Human Epidermal growth factor Receptor 4 (HER4 or ERBB4) carries out essential functions in the development and maintenance of the cardiovascular and nervous systems. HER4 activation is regulated by a diverse group of extracellular ligands including the neuregulin (NRG) family and betacellulin (BTC), which promote HER4 homodimerization or heterodimerization with other HER receptors. Important cardiovascular functions of HER4 are exerted via heterodimerization with its close homolog and orphan receptor, HER2. Here, we report cryo-EM structures of near full-length HER2/HER4 heterodimers and full-length HER4 homodimers bound to NRG1β and BTC.

We used this set of interface mutations to enrich for the fraction of functional HER2-G778D-V956R/HER4-I712Q heterodimers in large-scale purification for structural studies. Focused data processing on the ectodomains resulted in reconstructions of the NRG1β- and BTC-bound HER2/HER4 heterodimers at 3.3 Å and 4.3 Å resolution, respectively. We present here the first cryo-EM reconstructions of both the homodimer and heterodimer complexes of the HER4 receptor in its full-length form, bound to two different high-affinity HER4 cognate growth factors, NRG1β and BTC. This is also the first time that a betacellulin growth factor has been resolved bound to a HER receptor. Despite the diverse sequences of the NRG1β and BTC ligands, the larger-scale domain conformation of the HER2/HER4 heterodimers stabilized by each ligand is identical with only small differences in the ligand binding pockets. Due to the lower resolution of the HER2/HER4/BTC complex, we cannot exclude the possibility of differences in side-chain arrangements between the two structures. However, we attribute the lower resolution to variability in data collection on GO grids, rather than differences in conformational heterogeneity of HER2/HER4/BTC. HER2 and HER4 dimerization arms are resolved in both NRG1β and BTC-bound HER2/HER4 complexes. Extensive 3D variability and 3D classification analysis of the HER2/HER4/NRG1β and HER2/HER4/BTC datasets did not reveal any defined conformational heterogeneity within domains IV or dimerization arm regions. N-linked glycosylation is also resolved in the cryo-EM maps of the HER2/HER4 heterodimers (NRG1β and BTC bound), with HER4 glycosylation patterns being the same as seen in homodimers. However, in contrast to the HER4 homodimers, we do not observe continuous density connecting the two heterodimer monomers indicating that glycan-mediated interfaces seen in HER4 homodimers cannot be established in HER2/HER4 heterodimers.

> QSVCAGTENKLSSLSDLEQQYRALRKYYENCEVVMGNLEITSIEHNRDLSFLRSVREVTGYVLVALNQFRYLPLENLRIIRGTKLYEDRYALAIFLNYRKDGNFGLQELGLKNLTEILNGGVYVDQNKFLCYADTIHWQDIVRNPWPSNLTLVSTNGSSGCGRCHKSCTGRCWGPTENHCQTLTRTVCAEQCDGRCYGPYVSDCCHRECAGGCSGPKDTDCFACMNFNDSGACVTQCPQTFVYNPTTFQLEHNFNAKYTYGAFCVKKCPHNFVVDSSSCVRACPSSKMEVEENGIKMCKPCTDICPKACDGIGTGSLMSAQTVDSSNIDKFINCTKINGNLIFLVTGIHGDPYNAIEAIDPEKLNVFRTVREITGFLNIQSWPPNMTDFSVFSNLVTIGGRVLYSGLSLLILKQQGITSLQFQSLKEISAGNIYITDNSNLCYYHTINWTTLFSTINQRIVIRDNRKAENCTAEGMVCNHLCSSDGCWGPGPDQCLSCRRFSRGRICIESCNLYDGEFREFENGSICVECDPQCEKMEDGLLTCHGPGPDNCTKCSHFKDGPNCVEKCPDGLQGANSFIFKYADPDRECHPCHPNCTQGCNGPTSHDCI;> QVCTGTDMKLRLPASPETHLDMLRHLYQGCQVVQGNLELTYLPTNASLSFLQDIQEVQGYVLIAHNQVRQVPLQRLRIVRGTQLFEDNYALAVLDNGDPLNNTTPVTGASPGGLRELQLRSLTEILKGGVLIQRNPQLCYQDTILWKDIFHKNNQLALTLIDTNRSRACHPCSPMCKGSRCWGESSEDCQSLTRTVCAGGCARCKGPLPTDCCHEQCAAGCTGPKHSDCLACLHFNHSGICELHCPALVTYNTDTFESMPNPEGRYTFGASCVTACPYNYLSTDVGSCTLVCPLHNQEVTAEDGTQRCEKCSKPCARVCYGLGMEHLREVRAVTSANIQEFAGCKKIFGSLAFLPESFDGDPASNTAPLQPEQLQVFETLEEITGYLYISAWPDSLPDLSVFQNLQVIRGRILHNGAYSLTLQGLGISWLGLRSLRELGSGLALIHHNTHLCFVHTVPWDQLFRNPHQALLHTANRPEDECVGEGLACHQLCARGHCWGPGPTQCVNCSQFLRGQECVEECRVLQGLPREYVNARHCLPCHPECQPQNGSVTCFGPEADQCVACAHYKDPPFCVARCPSGVKPDLSYMPIWKFPDEEGACQPCPIN;> GHFSRCPKQYKHYCIKGRCRFVVAEQTPSCVCDEGYIGARCERVDLFY>[6x]MSSFSTQTPYPNLAVPFFTSIPNGLYPSKSIVIS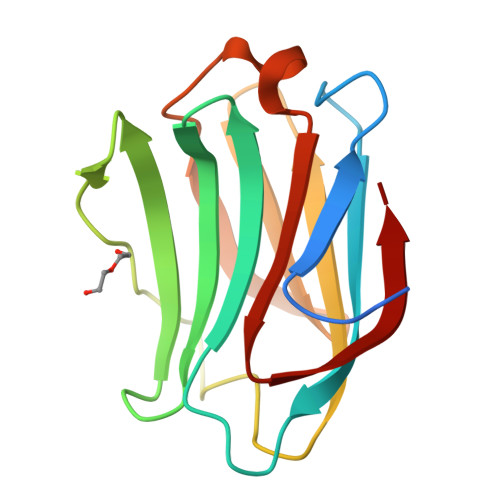GVVLSDAKRFQINLRCGGDIAFHLNPRFDENAVVRNTQINNSWGPEERSLPGSMPFSRGQRFSVWILCEGHCFKVAVDGQHICEYSHRLMNLPDINTLEVAGDIQLTHVET> GIPRNSRVDSDDFLWFEGIAFPTMGFRSETLRKVRDEFVIRDEDVIILTY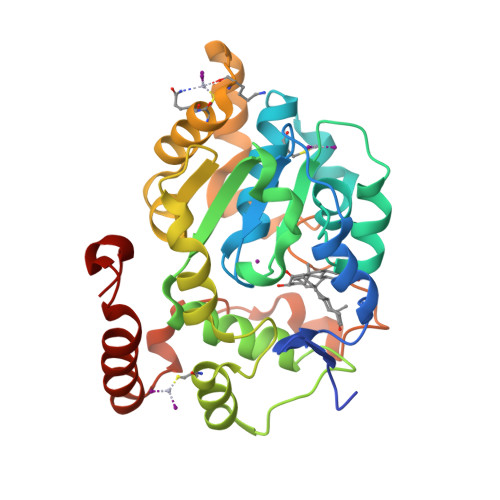PKSGTNWLAEILCLMHSKGDAKWIQSVPIWERSPWVESEIGYTALSETESPRLFSSHLPIQLFPKSFFSSKAKVIYLMRNPRDVLVSGYFFWKNMKFLKKPKSWEEYFEWFCQGTVLYGSWFDHIHGWMPMREEKNFLLLSYEELKQDTGRTIEKICQFLGKTLEPEELNLILKNSSFQSMKENKMSNYSLLSVDYVVDKTQLLRKGVSGDWKNHFTVAQAEDFDKLFQEKMADLPRELFPWE>SMAEDADMRNELEEMQRRADQLADESLESTRRMLQLVEESKDAGIRTLVMLDEQGEQLERIEEGMDQINKDMKEAEKNLTDLGK[2x];>[2x]MALSEIETRHSEIIKLENSIRELHDMFMDMAMLVESQGEMIDRIEYNVEHAVDYVERAVSDTKKAVKYQSKARRKKIM;>[4x]GMDTSGKQAEAMALLAEAERKVKNSQSFFSGLFGGSSKIEEACEIYARAANMFKMAKNWSAAGNAFCQAAQLHLQLQSKHDAATCFVDAGNAFKKADPQEAINCLMRAIEIYTDMGRFTIAAKHHISIAEIYETELVDVEKAIAHYEQSADYYKGEESNSSANKCLLKVAGYAAQLEQYQKAIDIYEQVGTSAMDSPLLKYSAKDYFFKAALCHFCIDMLNAKLAVQKYEELFPAFSDSRECKLMKKLLEAHEEQNVDSYTESVKEYDSISRLDQWLTTMLLRIKKTIQGDEEDLR;>[2x]GAHMAGRSMQAARCPTDELSLSNCAVVSEKDYQSGQHVIVRTSPNHKYIFTLRTHPSVVPGSVAFSLPQRKWAGLSIGQEIEVALYSFDKAKQCIGTMTIEIDFLQKKNIDSNPYDTDKMAAEFIQQFNNQAFSVGQQLVFSFNDKLFGLLVKDIEAMDPSILKGEPASGKRQKIEVGLVVGN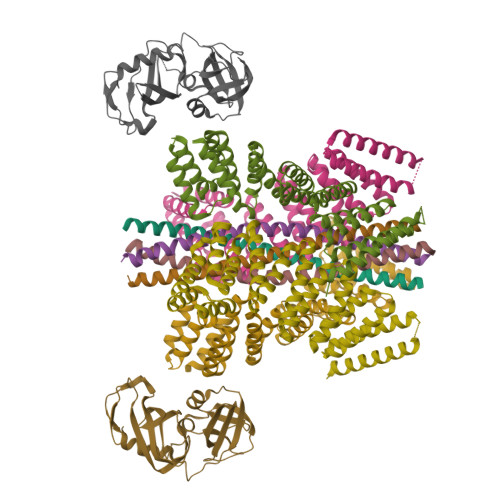SQVAFEKAENSSLNLIGKAKTKENRQSIINPDWNFEKMGIGGLDKEFSDIFRRAFASRVFPPEIVEQMGCKHVKGILLYGPPGCGKTLLARQIGKMLNAREPKVVNGPEILNKYVGESEANIRKLFADAEEEQRRLGANSGLHIIIFDEIDAICKQRGSMAGSTGVHDTVVNQLLSKIDGVEQLNNILVIGMTNRPDLIDEALLRPGRLEVKMEIGLPDEKGRLQILHIHTARMRGHQLLSADVDIKELAVETKNFSGAELEGLVRAAQSTAMNRHIKASTKVEVDMEKAESLQVTRGDFLASLENDIKPAFGTNQEDYASYIMNGIIKWGDPVTRVLDDGELLVQQTKNSDRTPLVSVLLEGPPHSGKTALAAKIAEESNFPFIKICSPDKMIGFSETAKCQAMKKIFDDAYKSQLSCVVVDDIERLLDYVPIGPRFSNLVLQALLVLLKKAPPQGRKLLIIGTTSRKDVLQEMEMLNAFSTTIHVPNIATGEQLLEALELLGNFKDKERTTIAQQVKGKKVWIGIKKLLMLIEMSLQMDPEYRVRKFLALLREEGASPLDFD> XGPPGPPGPPGPR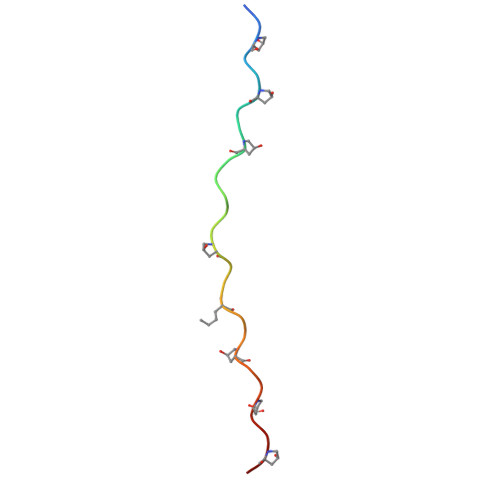GQPGVLGFPGPPGPPG>SGSGSTAEPDLKTALKAVIPAKRELFKQVKERSDEVIGEVKVANVIGGMRGLKSMLWEGSVLDPEEGIRFHGKTIKDCQKELPKGTSGTEMLPEAMFWLLLTGQVPSTNQVRAFSRELAEQSHLPQHILDLIKSFPRSMHPMTQLSIAVAALNTESKFAKAYEKGLSKADYWEPTFDDSISLLAKIPRVAALVFRPDEVDQVGTQALDASQDWSYNFAELLGKGGKENQDFHDLLRLYLALHGDHEGGNVSAHATHLVGSALSDPFLSYSAGLLGLAGPLHGLAAQEVLRWILAMQDKIGTKFTDDDVRNYLWDTLKSGRVVPGYGHGVLRKPDPRFQALMDFAATRPD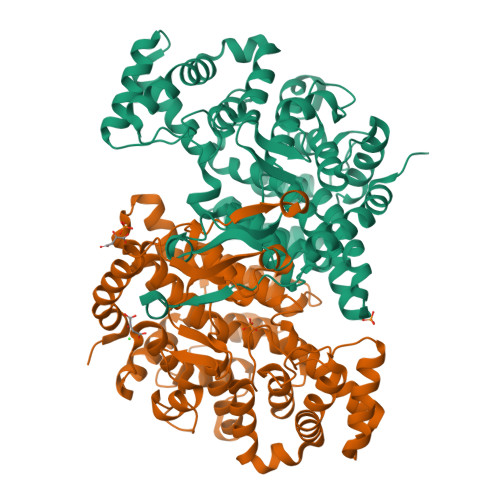VLANPVFQLVKKNSEIAPAVLTEHGKTKNPHPNVDAASGVLFYHYAFQQPLYYTVTFGVSRALGPLVQLIWDRALGLPIERPKSINLLGLKK[2x]> XCGGCGCC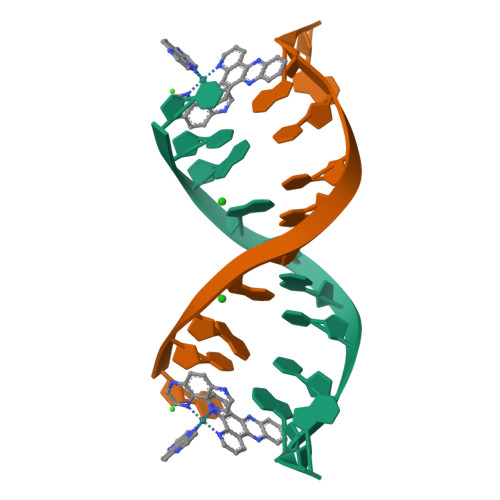GA> MVPISPIETVPVKLKPGMDGPKVKQWPLTEEKIKALVEICTEMEKEGKISKIGPENPYNTPVFAIKKKDSTKWRKLVDFRELNKRTQDFWEVQLGIPHPAGLPKKKSVTVLDVGDAYFSVPLDEDFRKYTAFTIPSINNETPGIRYQYNVLPQGWKGSPAIFQSSMTKILEPFAAQNPDIVIYQYMDDLYVGSDLEIGQHRTKIEELRQHLLRWGLTTPDKKHQKEPPFLWMGYELHPDKWTVQPIVLPEKDSWTVNDIQKLVGKLNWASQIYPGIKVRQLSKLLRGTKALTEVIPLTEEAELELAENREILKEPVHGVYYDPSKDLIAEIQKQGQGQWTYQIYQEPFKNLKTGKYARMRGAHTNDVKQLTEAVQKIT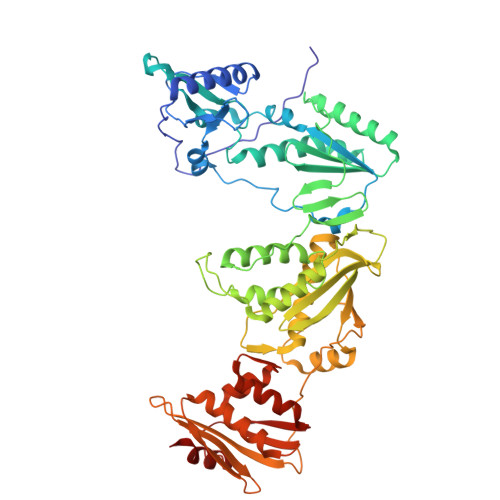TESIVIWGKTPKFKLPIQKETWETWWTEYWQATWIPEWEFVNTPPLVKLWYQLEKEPIVGAETFYVDGAANRETKLGKAGYVTNKGRQKVVPLTNTTNQKTELQAIYLALQDSGLEVNIVTDSQYALGIIQAQPDKSESELVNQIIEQLIKKEKVYLAWVPAHKGIGGNEQVDKLVSAG>SVGQRKQVNTNEKQVKVEKKEELTTSTVKKFLIAYYTKKDLGENRNRYEPLVTSAMYNELVNVEKQPVNQAYKGYVVNQVLDTYKIYIDTENNEVIVDVTYKNTQRTKRNNDEGALKNQSNQEALKLTFVKQGANFLVDKMAPVTLTNELQEE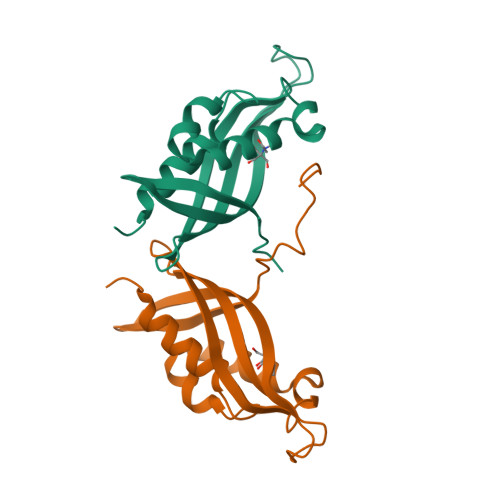PNSYNTHVVTTEESAKESANSGEKLEVLFQGPHHHHHHHHHH[2x]Rieske protein PetA, one of the three subunits of the bacterial cytochrome bc1 complex, functions as an electron transfer pathway in the photosynthesis of photosynthetic bacteria as well as in the respiration of aerobic bacteria. PetA has a hydrophilic globular domain containing one Rieske-type [2Fe-2S] cluster and a single transmembrane α-helix. The globular domain is exposed on the periplasmic side of the plasma membrane. TtPetA consists of two domains, an iron-sulfur cluster-binding domain and a large domain.

The structure of the Zn-containing form of a Rieske protein, in which ZnCl2 binds in the cluster-binding site, was determined. Diffraction data of the colorless TtPetA were collected at 1.7 Å resolution. Two monomers were observed in an asymmetric unit. An MX2-type compound appeared to bind in the cluster-binding site instead of the [2Fe-2S] type iron-sulfur cluster, judging from the electron density. On the other hand, no such densities were observed in the map of data collected at 1.29 Å, where the f” value of zinc was only 0.5e−. These observations provided confirmation that the element in the cluster-binding sites was actually zinc. The zinc ion has a tetra-coordination manner with two chloride ions in addition to two cysteine residues in the cluster-binding site of Zn-TtPetA. The zinc ion of ZnCl2 interacts with Sγ of Cys124 and Cys152 with distances of 2.4 Å and 2.3 Å, respectively. Probably due to the vacancy at this position, the side chain of His155 takes a different conformation mainly by a rotation around the Cβ−Cγ bond. Accordingly, the side chain of His155 has no interactions with ZnCl2. The Zn-containing structure indicates that the conformation of the cluster binding site is already constructed and stabilized before insertion of [2Fe-2S].

>[2x]PVEADISKLEPGALLRVKWRGKPVWLVHRTPEMLAALPSNDPKLVDPNSEVPQQPDYCKNPTRSIKPQYLVAIGICTHLGCSPTYRPEFGPDDLGADWKGGFFCPCHGSRFDLAARVFKNVPAPTNLVIPKHVYLNDTTILIGEDRGSA TRAF-interacting protein with a forkhead-associated (FHA) domain (TIFA) was originally identified as an adaptor protein that interacts with TRAF2 and TRAF61–3. TIFA has an FHA domain, involved in its binding to phosphothreonine (pThr), and has a consensus TRAF6-binding motif [PXEXX(Ar/Ac); Ar, aromatic; Ac, acidic; X, any] at the C-terminus for interaction with the TRAF-C domain of TRAF6 (TRAF6-C). Furthermore, oligomeric forms of TIFA promote oligomerisation and polyubiquitination of TRAF6, leading to the activation of IκB kinase (IKK). TIFA exists as an intrinsic dimer, and phosphorylation of TIFA at Thr9 promotes its oligomerisation through the intermolecular interaction of pThr9 with the FHA domain between the dimers.

Size-exclusion chromatography experiments of T9D/C36S and T9E/C36S showed that the phosphorylation-mimicking at Thr9 is partially involved in the TIFA assembly in solution (discussed later). Although it is difficult to discuss the original effect of pThr9 on oligomerisation even with the use of these results, the crystal structures of T9D/C36S and T9E/C36S provided structural insights into the assembly of TIFA. AB, A′1B′1, and A′2B′2 dimers assemble into a hexamer with a crystallographic three-fold symmetry due to interactions between adjacent dimers. The buried surface area per dimer in the hexamer formation is approximately 1,400 Å2. However, the buried surface area per dimer in tetramer formation (AB and CD dimers) is approximately 1,100 Å2, which is smaller than that in the TIFA hexamer. In hexamer formation, the adjacent AB and A′1B′1 dimers interact with each other at the interface between Mol AB and Mol B′1 through hydrogen bonds and van der Waals contacts. Glu39, Lys40, Glu45, and Gln57 (main chain) in Mol B, and Arg34, Ser37, Glu138, and Gln140 in Mol B′1 are involved in the interactions. The TIFA hexamer in the T9D/C36S crystal shows a large buried surface area of approximately 1,400 Å2 per dimer, and the interactions between the dimers are also observed in the crystal of T9E/C36S.

>MSTFEDADDEETVTCLQMTIYHPGQQSGIFKSIRFSSKEKFPSIEVVKFGRNSNMCQYTFQDKQVSRIQFVLQPFKQFNSSVLSFEIKNMSKKTSLMVDNQELGYLNKMDLPYKCMLRFGEYQFLLQKEDGESVESFETQFIMSSRPLLQENNWPTQNPIPEDGMYSSYFTHRSSPSEMDENELLEHHHHHH[4x]> MADYQGKNVVIIGLGLTGLSCVDFFLARGVTPRVMDTRMTPPGLDKLPEAVERHTGSLNDEWLMAADLIVASPGIALAHPSLSAAADAGIEIVGDIELFCREAQAPIVAITGSNGKSTVTTLVGEMAKAAGVNVGVGGN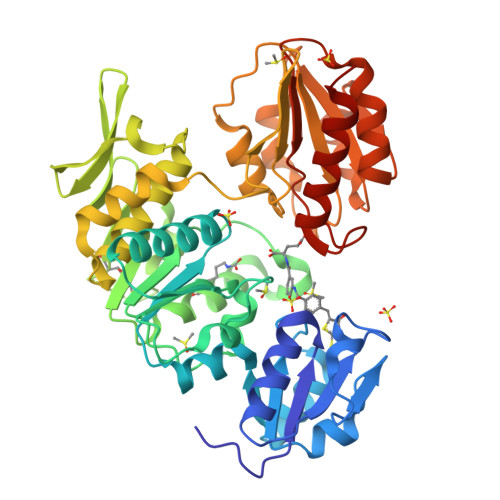IGLPALMLLDDECELYVLELSSFQLETTSSLQAVAATILNVTEDHMDRYPFGLQQYRAAKLRIYENAKVCVVNADDALTMPIRGADERCVSFGVNMGDYHLNHQQGETWLRVKGEKVLNVKEMKLSGQHNYTNALAALALADAAGLPRASSLKALTTFTGLPHRFEVVLEHNGVRWINDSKATNVGSTEAALNGLHVDGTLHLLLGGDGKSADFSPLARYLNGDNVRLYCFGRDGAQLAALRPEVAEQTETMEQAMRLLAPRVQPGDMVLLSPACASLDQFKNFEQRGNEFARLAKELGSHHHHHH> MTPLLELKDIRRSYPAGDEQVEVLKGISLDIYAGEMVAIVGASGSGKSTLMNILGCLDKATSGTYRVAGQDVATLDADALAQLRREHFGFIFQRYHLLSHLTAEQNVEVPAVYAGLERKQRLLRAQELLQRLGLEDRTEYYPAQLSGGQQQRVSIARALMNGGQVILADEPTGALDSHSGEEVMAILHQLRDRGHTVIIVTHDPQVAAQAERVIEIRDGEIVRNPPAIEKVNVTGGTEPVVNTVSGWRQFVSGFNEALTMAWRALAANKMRTLLTMLGIIIGIASVVSIVVVGD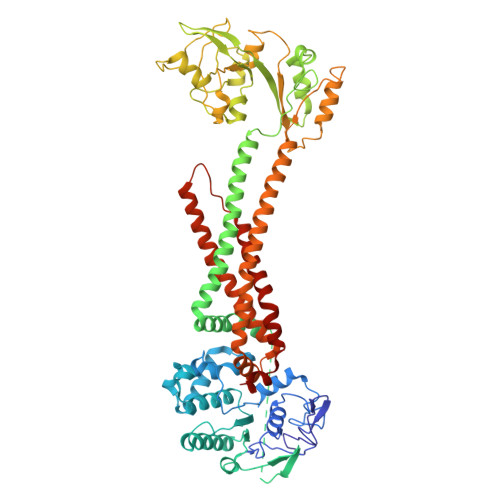AAKQMVLADIRSIGTNTIDVYPGKDFGDDDPQYQQALKYDDLIAIQKQPWVASATPAVSQNLRLRYNNVDVAASANGVSGDYFNVYGMTFSEGNTFNQEQLNGRAQVVVLDSNTRRQLFPHKADVVGEVILVGNMPARVIGVAEEKQSMFGSSKVLRVWLPYSTMSGRVMGQSWLNSITVRVKEGFDSAEAEQQLTRLLSLRHGKKDFFTWNMDGVLKTVEKTTRTLQLFLTLVAVISLVVGGIGVMNIMLVSVTERTREIGIRMAVGARASDVLQQFLIEAVLVCLVGGALGITLSLLIAFTLQLFLPGWEIGFSPLALLLAFLCSTVTGILFGWLPARNAARLDPVDALAREHHHHHH>[3x]MSSQFIFEDVPQRNAATFNPEVGYVAFIGKYGQQLNFGVARVFFLNQKKAKMVLHKTAQPSVDLTFGGVKFTVVNNHFPQYVSNPVPDNAITLHRMSGYLARWIADTCKASVLK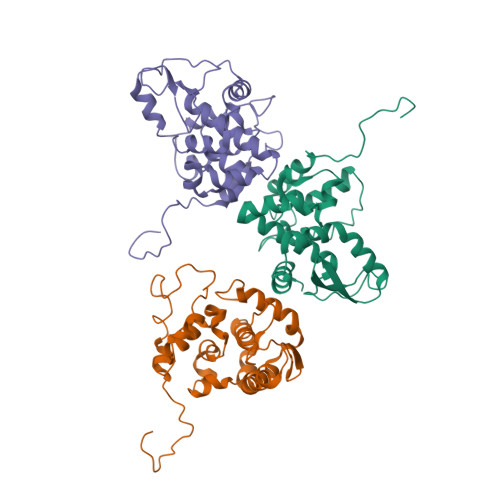LAEASAQIVMPLAEVKGCTWADGYTMYLGFAPGAEMFLDAFDFYPLVIEMHRVLKDNMDVNFMKKVLRQRYGTMTAEEWMTQKITEIKAAFNSVGQLAWAKSGFSPAARTFLQQFGINI(1R,2R,3R,4S,5R)-4-AMINO-5-(METHYLTHIO)CYCLOPENTANE-1,2,3-TRIOL | C6 H13 N O3 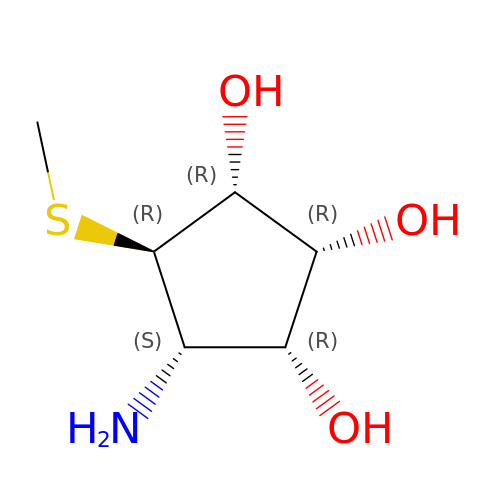S | BLOFGONIVNXZME-YDMGZANHSA-N> SNAACGGPSETKKDTAQNSKPIEITDVTGRTVTLKKPAERVVLQWSGAGGPFFTISALMGKDTPKVIAGMDTSLQDYRADMWKHFTAEMPELAKIPVVGTIGDKTFNAEQVVALNPDVIFIPVDLKDQYESDAKAKMDAAGIQTIYIDYHAEKLESHQKSIEAIGKALGKEERAAEISKFYTNRVTRVLDRVSKINKPKPTVYLEVGMNGPEEFGNSFSGNYSWGALATMAGA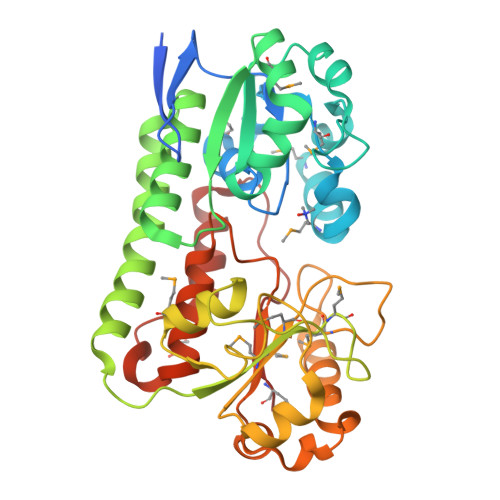DVITKDAIKKSSPINPEFVLEKNPDIIMIMGSYWPKKPTSMRLGFEATEDSSQALLKAFTTERQGWSDLKAVENKQVYSAHHGLPREVFDAAVFEYLAKTFYPEEFKDVDPEATLKEFYDKFLPFSYSGIWFMHMN> MNELVDTTEMYLRTIYDLE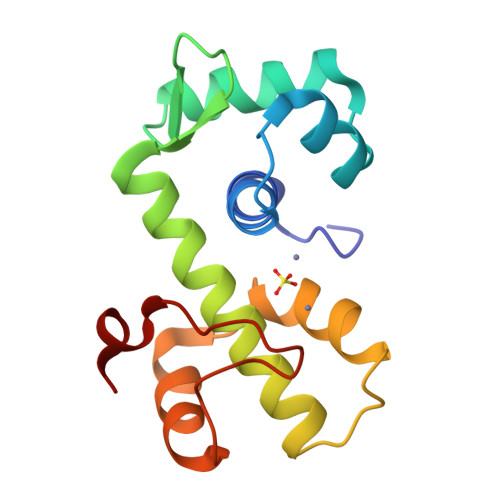EEGVTPLRARIAERLDQSGPTVSQTVSRMERDGLLRVAGDRHLELTEKGRALAIAVMRKHRLAERLLVDVIGLPWEEVHAEACRWEHVMSEDVERRLVKVLNNPTTSPFGNPIPGLVELGV> IPITVDFSGGLEMLFDNQRRHSISLPAKDTEGKPVTIAFLIDYICKKLMKDPRTDLFVLDNHIRPGILVLINDADWELEGEEAYEIQ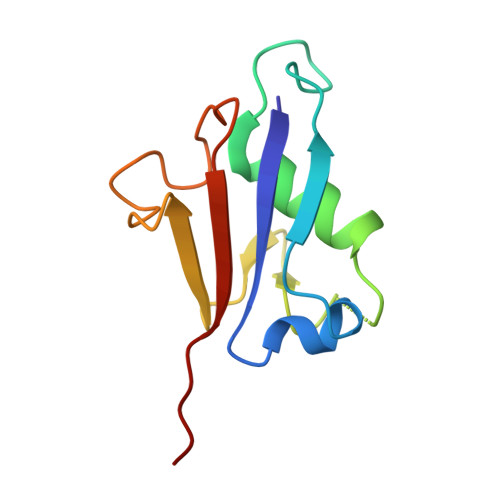PNDNILFVSTLHGG>MMSETAPLPSASSALEDKAASAPVVGIIMGSQSDWETMRHADALLTELEIPHETLIVSAHRTPDRLADYARTAAERGLNVIIAGAGGAAGLPGMCAAWTRLPVLGVPVESRALKGMDSLLSIVQMPGGVPVGTLAIGASGAKNAALLAASILALYNPALAARLETWRALQTASVPNS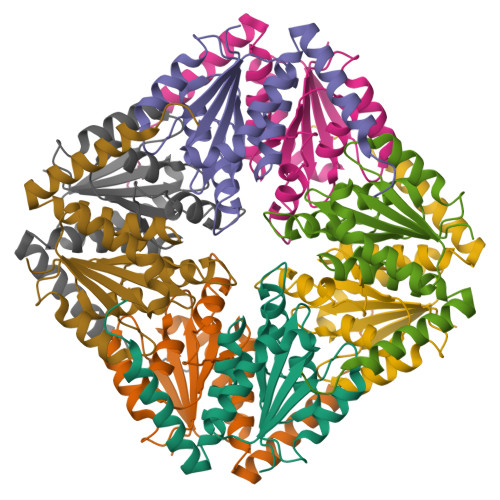PITEDK[2x]>MHHHHHHSSGRENLYFQGSRKEMTAACTPRRRIINLTSVLSLQEEINEQGHEVLREMLHNHSFVGCVNPQWALAQHQTKLYLLNTTKLSEELFYQILIYDFANFGVLRLSEPAPLFDLAMLALDSPESGWTEEDGPKEGLAEYIVEFLKKKAEMLADYFSLEIDEEGN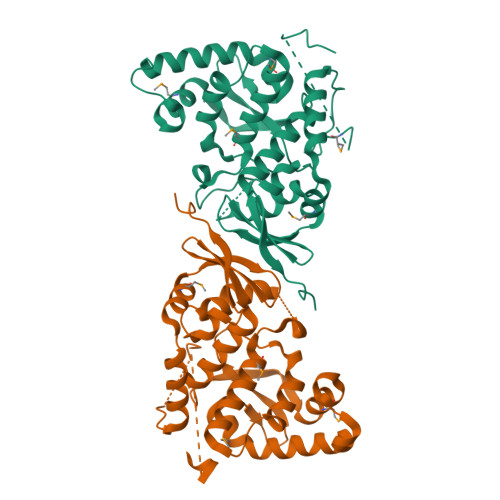LIGLPLLIDNYVPPLEGLPIFILRLATEVNWDEEKECFESLSKECAMFYSIRKQYISEESTLSGQQSEVPGSIPNSWKWTVEHIVYKALRSHILPPKHFTEDGNILQLANLPDLYK[2x]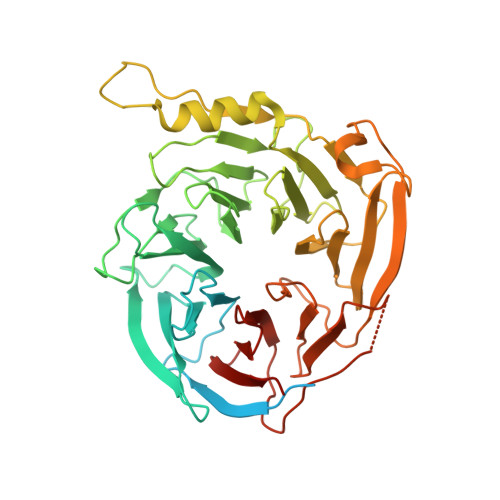> MSSEREVSTAPAGTDMPAAKKQKLSSDENSNPDLSGDENDDAVSIESGTNTERPDTPTNTPNAPGRKSWGKGKWKSKKCKYSFKCVNSLKEDHNQPLFGVQFNWHSKEGDPLVFATVGSNRVTLYECHSQGEIRLLQSYVDADADENFYTCAWTYDSNTSHPLLAVAGSRGIIRIINPITMQCIKHYVGHGNAINELKFHPRDPNLLLSVSKDHALRLWNIQTDTLVAIFGGVEGHRDEVLSADYDLLGEKIMSCGMDHSLKLWRINSKRMMNAIKESYDYNPNKTNRPFISQKIHFPDFSTRDIHRNYVDCVRWLGDLILSKSCENAIVCWKPGKMEDDIDKIKPSESNVTILGRFDYSQCDIWYMRFSMDFWQKMLALGNQVGKLYVWDLEVEDPHKAKCTTLTHHKCGAAIRQTSFSRDSSILIAVCDDASIWRWDRLR2-(2-HYDROXY-1,1-DIHYDROXYMETHYL-ETHYLAMINO)-ETHANESULFONIC 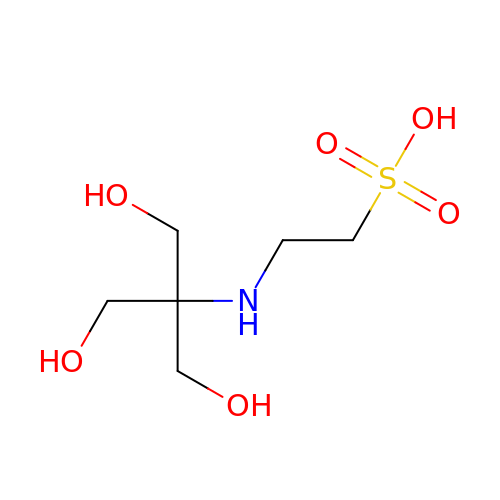ACID | C6 H15 N O6 S | JOCBASBOOFNAJA-UHFFFAOYSA-N> MGLLTILKKMKQKERELRLLMLGLDNAGKTTILKKFNGEDIDTISPTLGFNIKTLEHRGFKLNIWDVGGQKSLRSYWRNYFESTDGLIWVVDSADRQRMQDCQRELQSLLVEERLAGATLLI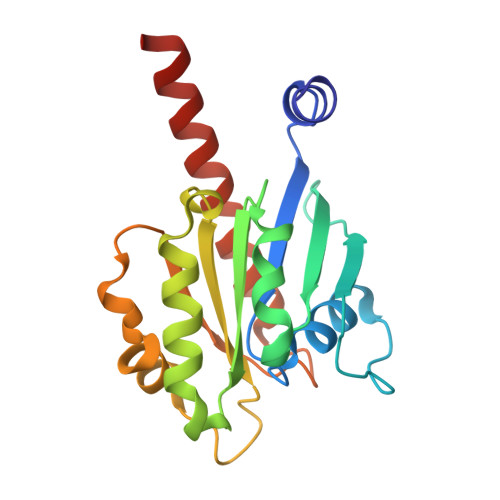FANKQDLPGALSSNAIREVLELDSIRSHHWCIQGCSAVTGENLLPGIDWLLDDISSRIFTADLEHHHHHH> MFILSKIADLVRIPPDQFHRDTISAITHQLNNKFANKIIPNVGLCITIYDLLTVEEGQLKPGDGSSYINVTFRAVVFKPFLGEIVTGWISKCTAEGIKVSLLGIFDDIFIPQNMLFEGCYYTPEESAWIWPMDEETKLYFDVNEKIRFRIEREVFVDVKPKSPKERELEERAQLENEIEGKNEETPQNEKPPAYALLG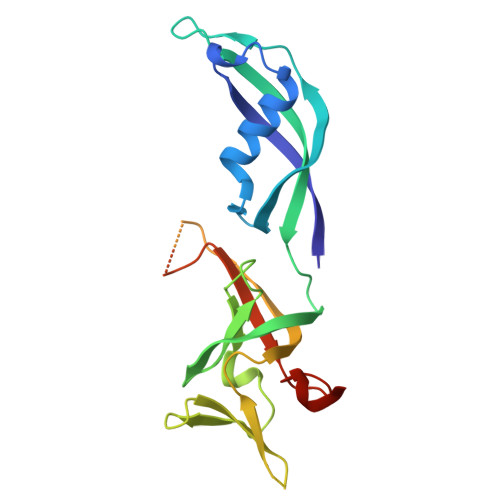SCQTDGMGLVSWWEHHHHHH>MHHHHHHMKSIDEQSLHNARRLFESGDIDRIEVGTTAGLQQIHRYLFGGLYDFAGQIREDNISKGGFRF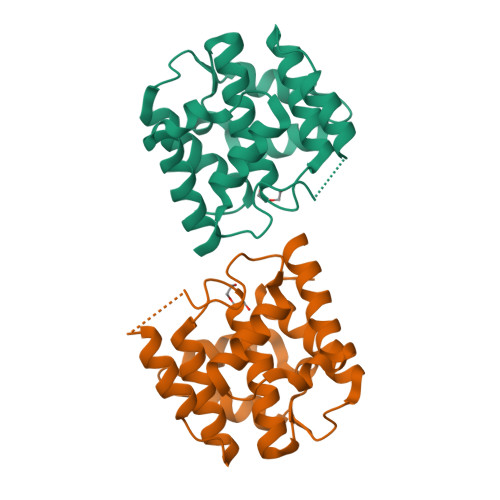ANAMYLKEALVKIEQMPERTFEEIIAKYVRMNIAHPFLEGNGRSTRIWLDLVLKKNLKKVVNWQNVSKTLYLQAMERSPVNDLELRFLLKDNLTDDVDNREIIFKGIEQSYYYEGYEKG[2x]>[2x]GAELPAPLRRTGVGEWLATTCQGCTSWCAKQIYVMDGRALKVRGNPNSGVHGMSSCPRQHLSLQQVYDPDRLRTPMMRTNPKKGRDQDPKFVPISWDKALDMLADKIIALRVANEPHKYALLRGRYSHINDLLYKKMTNLIGSPNNISHSSVCAEAHKMGPYYLDGNWGYNQYDVKNAKFILSFGADPIASNRQVSFYSQTWGDSLDHAKVVVVDPRLSASAAKAHKWIPIEPGQDSVLALAIAHVALVEGVWHKPFVGDFIEGKNLFKAGKTVSVESFKETHTYGLVEWWNQALKDYTPEWASKITGIDPKTIIAIAKDMGAAAPAVQVWTSRGAVMQARGTYTSISCHALNGLFGGIDSKGGLFPGNKTPLLKEYPEAKAYMDEIAAKGVKKEKIDQRGRLEFPALAKGKSGGGVITANAANGIRNQDPYEIKVMLAYFNNFNFSNPEGQRWDEALSKVDFMAHITTNVSEFSWFADVLLPSSHHMFEKWGVLDSIGNGVAQISIQQPSIKRLWDTRIDESEIPYMLAKKLADKGFDAPWRYINEQIVDPETGKPAADEAEFAKLMVRYLTAPLWKEDASKYGDKLSSWDEFVQKGVWNSSPYKLEARWGKFKTETTKFEFYSKTLEKALQSHADKHKVSIDEVMKACDYQARGHLAFIPHYEEPYRFGDESEFPLLLVDQKSRLNKEGRTANSPWYYEFKDVDPGDVANEDVAKFNPIDGKKFGLKDGDEIRITSPVGMLTCKAKLWEGVRPGTVAKCFGQGHWAYGRYASAKFGVTPRGGSNNDLIADRYDRLSGASAFYGHIRVRVEKV;>[2x]MRLGMVIDLQKCVGCGGCSLACKTENNTNDGIH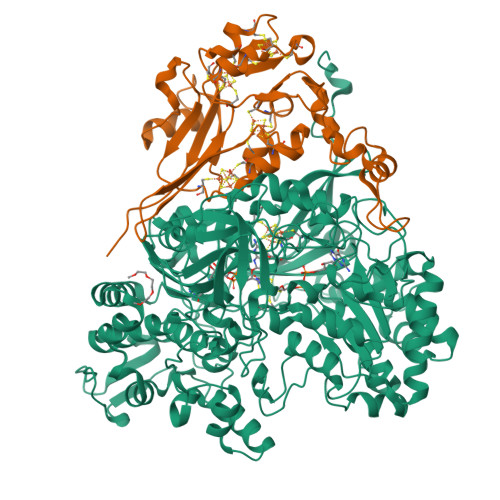WSHHIATTEGTFPDVKYTYIPTLCNHCDDAPCVKVCPTGAMHKDKRGLTLQNNDECIGCKKCMNACPYGVISFNAATPHRRWQDDSEVVANGTVSPLMLLKRTGATATPNENPERGDTYPMIRPKRTTEKCTFCDHRLDKGLNPACVDACPSEARVIGDLDDPQSKVSQLIKLHKPMQLKPEAGTGPRVFYIRSFGVKTAY>NTTSSVILTNYMDTQYYGEIGIGTPPQT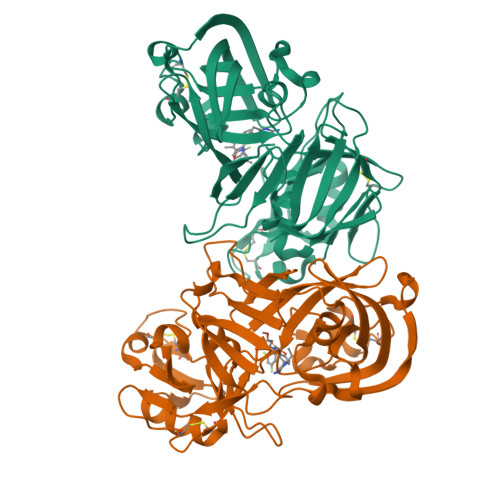FKVVFDTGSSNVWVPSSKCSRLYTACVYHKLFDASDSSSYKHNGTELTLRYSTGTVSGFLSQDIITVGGITVTQMFGEVTEMPALPFMLAEFDGVVGMGFIEQAIGRVTPIFDNIISQGVLKEDVFSFYYNRDSENSQSLGGQIVLGGSDPQHYEGNFHYINLIKTGVWQIQMKGVSVGSSTLLCEDGCLALVDTGASYISGSTSSIEKLMEALGAKKRLFDYVVKCNEGPTLPDISFHLGGKEYTLTSADYVFQESYSSKKLCTLAIHAMDIPPPTGPTWALGATFIRKFYTEFDRRNNRIGFALAR[2x]>QYSPNTQQGRTSIVHLFEWRWVDIALECERYLAPKGFGGVQVSPPNENVAIYNPFRPWWERYQPVSYKLCTRSGNEDEFRNMVTRCNNVGVRIYVDAVINHMCGNAVSAGTSSTCGSYFNPGSRDFPAVPYSGWDFNDGKCKTGSGDIENYNDATQVRDCRLTGLLDLALEKDYVRSKIAEYMNHLIDIGVAGFRLDASKHMWPGDIKAILDKLHNLNSNWFPAGSKPFIYQEVIDLGGEPIKSSDYFGNGRVTEFKYGAKLGTVIRKWNGEKMSYLKNWGEGWGFVPSDRALVFVDNHDNQRGHGAGGASILTFWDARLYKMAVGFMLAHPYGFTRVMSSYRWPRQFQNGNDVNDWVGPPNNNGVIKEVTINPDTTCGNDWVCEHRWRQIRNMVIFRNVVDGQPFTNWYDNGSNQVAFGRGNRGFIVFNNDDWSFSLTLQTGLPAGTYCDVISGDKINGNCTGIKIYVSDDGKAHFSISNSAEDPFIAIHAESKL[2x];>XYGHSHIRFGYSYHVSY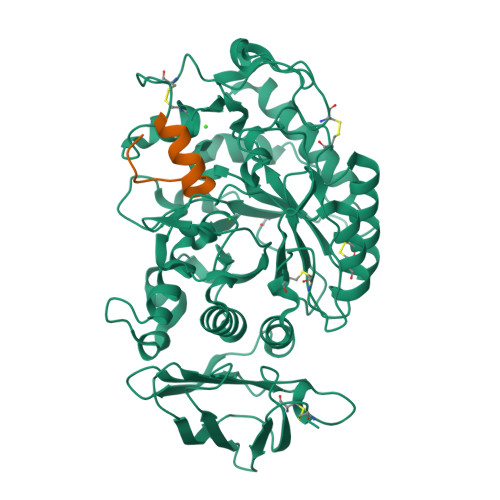CGX[2x]> GSSAKRKQEEKHLKMLRDMTGLPHNRKCFDCDQRGPTYVNMTVGSFVCTSCSGSLRGLNPPHRVKSISMTTFTQQEIEFLQKHGNEVCKQIWLGLFDDRSSAIPDFRDPQKVKEFLQEK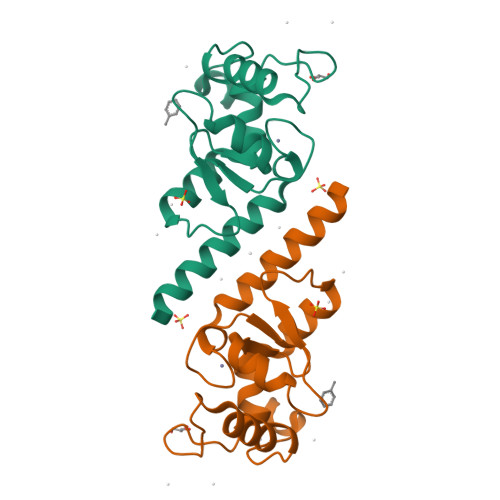YEKKRWYVPPEQAKVVASVHA>[2x]MNTTPVHALTDIDGGIAVDPAPRLAGPPVFGGPGNDAFDLAPVRSTGREMLRFDFPGVSIGAAHYEEGPTGATVIH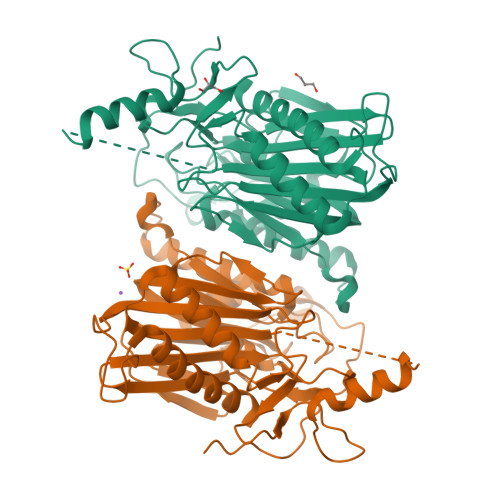IPAGARTAVDARGGAVGLSGGYDFNHAICLAGGAGYGLEAGAGVSGALLERLEYRTGFAELQLVSSAVIYDFSARSTAVYPDKALGRAALEFAVPGEFPQGRAGAGMSASAGKVDWDRTEITGQGAAFRRLGDVRILAVVVPNPVGVIVDRAGTVVRGNYDAQTGVRRHPVFDYQEAFAEQVPPVTEAGNTTISAIVTNVRMSPVELNQFAKQVHSSMHRGIQPFHTDMDGDTLFAVTTDEIDLPTTPGSSRGRLSVNATALGAIASEVMWDAVLEAGK> GGCUUAUCAAGAGAGGUUUAGGGACUGGCCCGACGAAACCCGGCAACCAGAAAUGGUGCCAAUUCCUGCAGCGGAAACGUUGAAAGAUGAGCCG

The SAM-I riboswitch contains an essential standard k-turn sequence that kinks a helix so that its terminal loop can make a long-range interaction. The SAM-I riboswitch is based around an elaborated four way helical junction; the crystal structure of the SAM-I riboswitch of Thermoanaerobacter tengcongensis was solved by Batey and colleagues, showing that the junction creates a pocket for the binding of SAM. Two adjacent helical arms of the junction make a tertiary contact in which the terminal loop of one helix (P2) base pairs with an internal loop within the other (P4). In order to do this, helix P2 must be severely kinked, and this is facilitated by a k-turn.

We have also solved the crystal structure for the SAM-I riboswitch in which the k-turn contains the double G2nU, G3nU substitution. As with the G2nA, this intrinsically unstable k-turn is stabilized in the context of the riboswitch. We have also analyzed the double substitution G2nU, G3nU in the context of the complete riboswitch, which was titrated with SAM. The corresponding binding affinity Kd = 1.95 ± 0.27 μM is about 4-fold weaker than that of the natural riboswitch. Nevertheless, this double substitution that prevented the folding of the isolated k-turn is tolerated in the context of the riboswitch. The crystals diffracted to 2.9 Å, but due to low completeness between 2.9 and 3.0 Å the data set is regarded as 3 Å resolution. The overall fold and structure of the riboswitch is again maintained, with an rmsd from the natural riboswitch of <0.5 Å, the k-turn regions of the natural and variant riboswitches superimposed with an rmsd of 0.75 Å, showing that the global structure of the k-turn was preserved in the riboswitch. However, while the complete backbone of the G2nU, G3nU k-turn structure is well defined by the electron density, some of the nucleobases in the core of the structure are relatively weakly defined at this resolution, including the two uridine bases at the 2n and 3n positions, i.e., the two substituted nucleotides. In principle, an A⋅U pair could form at the 2b⋅2n position of the G2nU, G3nU variant, but we cannot be sure that it does so on the basis of the present structure for that riboswitch.> G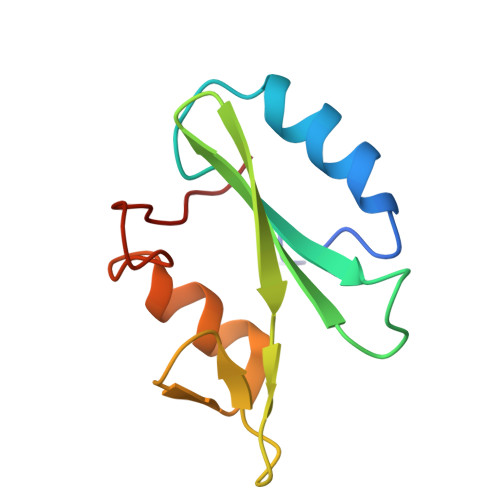SMAWFFGKIPRAKAEEMLSKQRHDGAFLIRESESAPGDFSLSVKFGNDVQHFKVLRDGAGKYFLWVVKFNSLNELVDYHRSTSVSRNQQIFLRDI>QMQKEQLNLMPWPQNVVVNDGNFTLTKNFKVNISGNPDSRIFGGVTRFLRRLDGRTGIFFEQGFITKLNEFPNAELQINCTKNGKIGLYEDESYSLDVKANKITINATSDLGALHGLETLLQLLQNDSKKFYFPVSQISDFPRFTWRGLMLDASRHFQPVDVVKRNLDALAAMKMNVFHWHLVDDQGWRIETKKHPKLIELASDGLYYTQEEIRNIVKYADERGILIVPEIDVPGHGSAILTAYPEIGSKVITLTGGTSEKNIQGTAISTYRIERNAGIFSPTLDPSNPKTYKILSELFDEVCPLFPGAYFHIGGDENEGKDWDANPKIQEFKKKHNLKTNHELQTY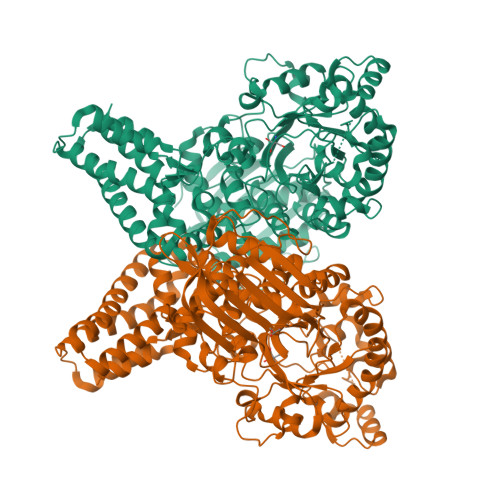FTMQLAPMLKKHGKQLMGWEEILTKDLSKEAIVHSWRGPNEGMVAGQSLVDAVKKGYKTVLSNGFYIDLMYPVASHYLNDPMPKGADLSAEEKARILGGEATMWTELATPETFDSRVWPRTAAIAERLWSAENITDVANMRKRLESVSFRLEELGLTHIKNKAVILRNIANNQNIKSVNEFTNVCEPLKGYTRNKGGTEYQMYSPFTLFADACTPDAKDSLAFDEAVSQYLANKSADNKAKVAAFFNKWIAVNKGLVELSANAPLVQPILPLSKKLSDASQELLLVLDNKSTLKTADLKTLIEQCNTKDHADVELSVYESLKKLIA[2x]>GPATSPTDEAKGHTGIGELAAALNEFDNKIILDPMTFSEARFRPSLEERLESIISGAALMADSSCTRDDRRERIVAECNAVRQALQDLLSEYMNNTGRKEKGDPLNIAIDKMTKKTRDLRRQLRKAVMDHISDSFLETNVPLLVLIEAAKSGNEKEVKEYAQVFREHANKLVEVANLACSISNNEEGVKLVRMAATQIDSLCPQVINAALTLAARPQSKVAQDNMDVFKDQWEKQVRVLTEAVDDITS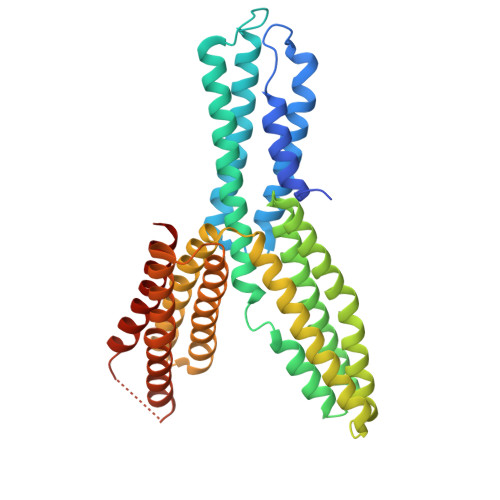VDDFLSVSENHILEDVNKCVIALQEGDVDTLDRTAGAIRGRAARVIHIINAEMENYEAGVYTEKVLEATKLLSETVMPRFAEQVEVAIEALSANVPQPFEENEFIDASRLVYDGVRDIRKAVLMIRT[4x]>[2x]GPLGSPEFGRPGWVIGVDPDIGGAIAVLSPDGSSQVFDNPFVHIVVSEVIRKRL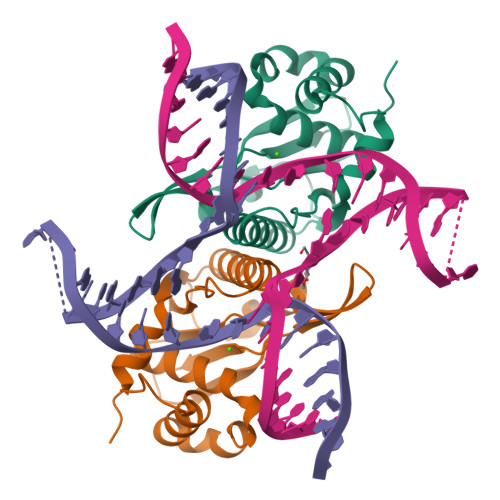DTKSIIQLLRGLDAPPGTTAYIEKSSPFPTDGKQGWWSTGFSYGLWIASLVASGFSVVPIASQTWKAYFGLMRSETPKDDSRQAASILFPDKDQSLKLKKHHGRAEALLLAAYGKGLVLP The amino acid transporter SLC38A9 is identified to be a lysosome-based arginine sensor for mTORC1, and the ACT [Pfam 01842; a small regulatory domain found in Aspartate kinase, Chorismate mutase and TyrA (prephenate dehydrogenase)] domain-containing protein CASTOR1 is a cytoplasm-localized arginine sensor. Similar to the regulation mechanism of Sestrin2 with GATOR2, CASTOR1 can also inhibit the GATOR2–GATOR1 mediated mTORC1 activation in starving cells; and the binding of arginine to CASTOR1 disrupts the CASTOR1–GATOR2 interaction and hence GATOR2 is released to form the GATOR1–GATOR2 complex, leading to the inhibition of GATOR1. The structure of CASTOR1 shows it composed of four tandem ACT domains (ACT1-4). The recombinant CASTOR1 protein exists as a homodimer in solution as revealed by gel filtration and dynamic light scattering analyses, and the dimerization is independent of arginine.

The structure of the arginine-bound CASTOR1 was solved by the single-wavelength anomalous dispersion method and was refined to 2.5 Å resolution, yielding an R-factor of 17.5% and a free R-factor of 22.4%. There are four arginine-bound CASTOR1 molecules in an asymmetric unit, forming two CASTOR1 homodimers which have almost identical overall structure with a root-mean-square deviation of 0.9 Å for 570 Cα atoms. However, ACT1 and ACT3 fold together to form an 8-stranded β-sheet flanked by four α-helices on one side, and ACT2 and ACT4 fold together to form a 10-stranded β-sheet flanked by four α-helices on the other side, and the two β-sheets are orthogonal to each other and form a β-barrel-like core which is sandwiched by the two layers of α-helices. In the structure of CASTOR1, two CASTOR1 molecules form a tight homodimer via a twofold non-crystallographic symmetry. The homodimer interface is stabilized by largely hydrophobic interactions and a few hydrogen-bonding interactions among residues from helices α1 of ACT1 and α5 of ACT3 of each monomer, which buries 1 857 Å2 or 7.1% of the total solvent accessible surface area as analyzed by the PISA server. In the structure of CASTOR1, arginine binds to the interface of the ACT2 and ACT4 domains with well-defined electron density and reasonable B-factor. The arginine-binding pocket is largely formed by residues from α7, the β17-β18 loop and β18 of ACT4 and the α3-β7 loop of ACT2, and additionally the β16-α7 loop (residues 269–279) acts as a lid to conceal the binding pocket. In detail, the α-carboxyl group of arginine forms four hydrogen bonds with the main chains of Val112, Gly279, Ile280 and Val281; and the α-amino group forms three hydrogen bonds with the side chain of Ser111 and the main chains of Val112 and Glu277. The guanidinium group forms five hydrogen bonds with the main chains of Gly274, Thr300, Phe301 and Phe303, and additionally makes a salt bridge with the side chain of Asp304.

>[4x]MELHILEHRVRVLSVARPGLWLYTHPLIKLLFLPRRSRCKFFSLTETPEDYTLMVDEEGFKELPPSEFLQVAEATWLVLNVSSHSGAAVQAAGVTKIARSVIAPLAEHHVSVLMLSTYQTDFILVREQDLSVVIHTLAQEFDIYREVGGEPVPVTRDDSSNGFPRTQHGPSPTVHPIQSPQNRFCVLTLDPETLPAIATTLIDVLFYSHSTPKEAASSSPEPSSITFFAFSLIEGYISIVMDAETQKKFPSDLLLTSSSGELWRMVRIGGQPLGFDECGIVAQIAGPLAAADISAYYISTFNFDHALVPEDGIGSVIEVLQRRQEGLASLEHHHHHH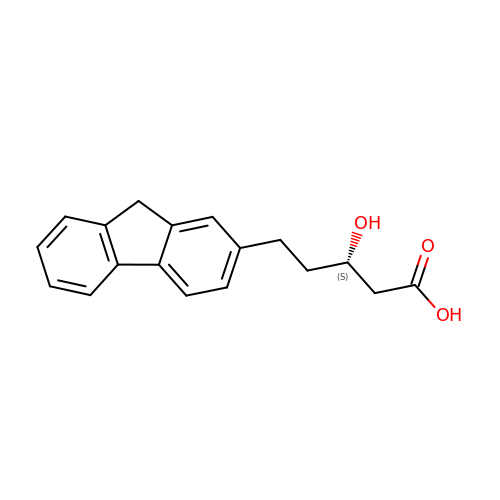(3S)-5-(9H-FLUOREN-2-YL)-3-HYDROXYPENTANOIC ACID | C18 H18 O3 | QNNGXIOOEUXOPM-HNNXBMFYSA-N>MKETAAAKFERQHMDSSTSAASSSNYCNQMMKSRNLTKDRCKPVNTFVHESLADVQAVCSQKN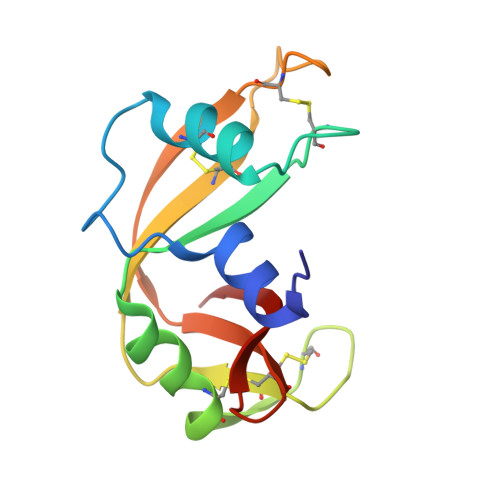VACKNGQTNCYQSYSTMSITDCRETGSSKYPNCAYKTTQANKHIIVGCEGNPYVPVHFDASV[2x]> AMGSMSTAAPAPGSTATVRVSNIPASAIAAELLAFFDSAVTIAGATFACEIVAAHRGWLSRGHGFVQFDSSAAATHAIDLASSGRLPPFLGSCLSVSPARADLLPRAPDLSLRAASASLILGNRVAERELEVAYSCDGVRAEVIPRMRRVDLYLKHDSQSYKLEVLFEDINECFGCHLDGTGAILLQLTYAPRIHIAISGSTVKSRFTDDRFHACKEDAKFAWVRALDFTPNSSFGECSTLVLKLSKGASVSYILESLPFSGELGELAIASMDVFGSSSNVVPLVDCPNGFSVPYEVLFRLNSLVHMGKLVARHVNADLFKVLEDLSIDTLRRIFEKMSKLKSTCYEPLQFIRHEAHSMNMRKKALSNKRESGKLMRCYRIHITPSKIYCLGPEEEVSNYVVKYHSEYASDFARVTFVDEDWSKLSPNALSARTEQGFFSKPLKTGLYHRILSILKEGFCIGPKKYEFLAFSASQLRGNSVWMFASNSSLTAENIRRWMGHFEDIRSVSKCAARMGQLFSSSRQTFEVSSYDVEVIPDIEVTTDGTKYIFSDGIGKISTRFARQVAKLIGLDPAHPPSAFQIRYGGYKGVITIDPTSFFNLSLRPSMKKFESKSTMLNITNWSKSQPCYVNREIISLLSTLGIKDEVFESMQQDDMHESDGMLTNKEAALSVLGKIGGGDTKTAADMLLQGYEPSSEPYLLMILKAHRANRLTDIRTRCKIHVQKGRVLIGCLDETCKLEYGQVYIRITKNHKEQKYSEQPFFCNDDGKTAVIVGKVAITKNPCLHPGDVRVLEAVYDPGLDARGLIDCVVFPQRGERPHPNECSGGDLDGDLFFITWDDKLIPEKVDAPMDYTATRPRIMDHAVTLEEIQKHFVSYMINDTLGAISTAHLIHADRDPLKARSPECVQLAALHSMAVDFAKTGAPAEMPLALRPREFPDFMERWERPMYVSNGVLGKLYRAALRHAADAAALLPAGPPSCVYDPDLEVAGFDEFLDAAEERYEAYAERLGALMTYYSAEREDEILTG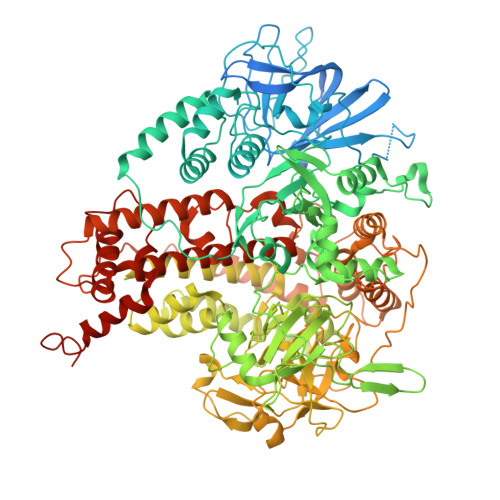NIRNKLVYLRRDNKRYFEMKDRIIAAVDALHAEVRGWLRACKEDDASRVASAWYHVTYHPDRRGEKRFWSFPWIICDTLLAIKAARRCRKRVEDAAVPMDCDGS> GPHMASTVSQMVDNVLSQPEGKRLMLLAPIIKERKGEHTKTLENLASQGYIRARIDGEVCDLSDPPKLELQKKHTIEVVVDRFKVRDDLTQRLAESFETALELSGGTAVVADMDDPKAEEL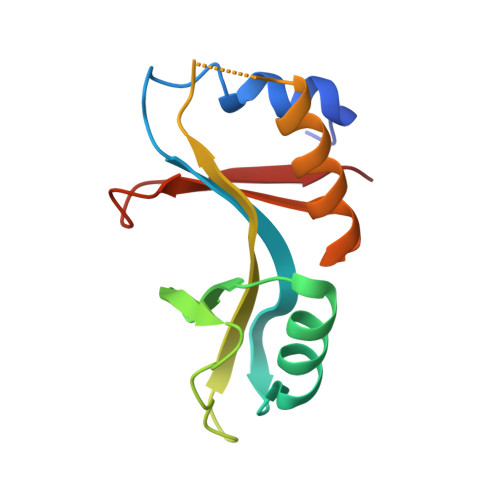LFSAN> SVVVQLTLAFREGTINVHDVETQFNQYKTEAASRYNLTISDVSVSDV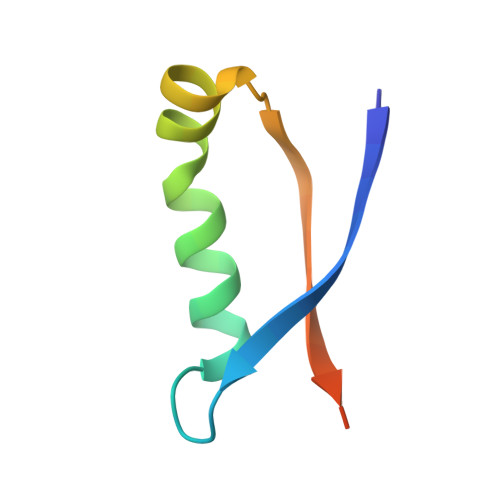PFPFSAQS>MSLQVEEVRISLPHIELAAHLFGPPDGKPVIALHGWLDNAMSFSRLAPKLAGLRIVALDFAGHGHSAHRAEGASYLLWDYALDVLMVAEQLGWERFSLLGHSMGAIVSVLLAGALPERIERLALIDGLIPYTGEADKAPQKLGEA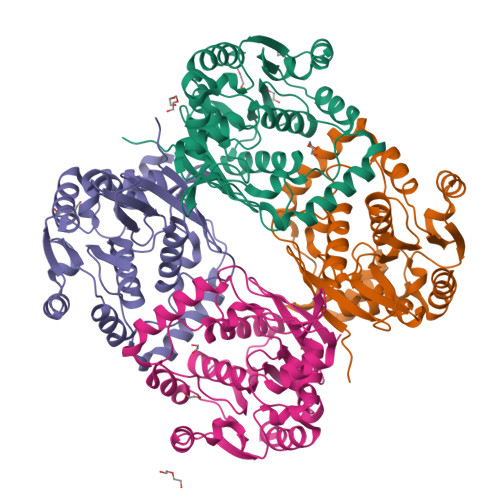LKAQLALRHKRKPVYAELEKAVEARMRGVGEISREAAELLAQRGLEPVPGGYTWRTDARLTLPSPLRLTQAHALNFVRSVECPVSLVLAEQGMLAVEPRMRALLETLPFERHHLPGGHHLHLDDEAGAQAVARVFAAFFAR[4x]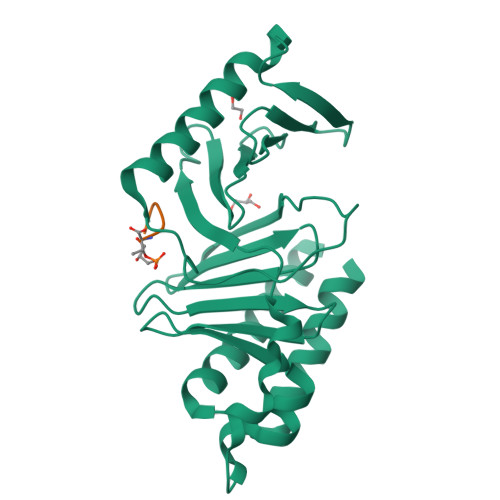> GEVVDCHLSDMLQQLHSVNASKPSERGLVRQEEAEDPACIPIFWVSKWVDYSDKYGLGYQLCDNSVGVLFNDSTRLILYNDGDSLQYIERDGTESYLTVSSHPNSLMKKITLLKYFRNYMSEHLLKAGANITPREGDELARLPYLRTWFRTRSAIILHLSNGSVQINFFQDHTKLILCPLMAAVTYIDEKRDFRTYRLSLLEEYGCCKELASRLRYARTMVDKLLSSRSASNRLKAS;> XPLHST> QRAKVAMSHFEPHEYIRYDLLEKNIDIVRKRLNRPLTLSEKIVYGHLDDPANQEIERGKTYLRLRPDRVAMQDATAQMAMLQFISSGLPKVAVPSTIHCDHLIEAQLGGEKDLRRAKDINQEVYNFLATAGAKYGVGFWRPGSGIIHQIILENYAYPGVLLIGTDSHTPNGGGLGGICIGVGGADAVDVMAGIPWELKCPKVIGVKLTGSLSGWTSPKDVILKVAGILTVKGGTGAIVEYHGPGVDSISCTGMATICNMGAEIGATTSVFPYNHRMKKYLSKTGRADIANLADEFKDHLVPDSGCHYDQLIEINLSELKPHINGPFTPDLAHPVAEVGSVAEKEGWPLDIRVGLIGSCTNSSYEDMGRSAAVAKQALAHGLKCKSQFTITPGSEQIRATIERDGYAQVLRDVGGIVLANACGPCIGQWDRKDIKKGEKNTIVTSYNRNFTGRNDANPETHAFVTSPEIVTALAIAGTLKFNPETDFLTGKDGKKFKLEAPDADELPRAEFDPGQDTYQHPPKDSSGQRVDVSPTSQRLQLLEPFDKWDGKDLEDLQILIKVKGKCTTDHISAAGPWLKFRGHLDNISNNLLIGAINSENRKANSVRNAVTQEFGPVPDTARYYKQHGIRWVVIGDENYGEGSSREHRALEPRFLGGRAIITKSFARIHETNLKKQGLLPLTFADPADYNKIHPVDKLTIQGLKDFAPGKPLTCIIKHPNGTQETILLNHTFNETQIEWF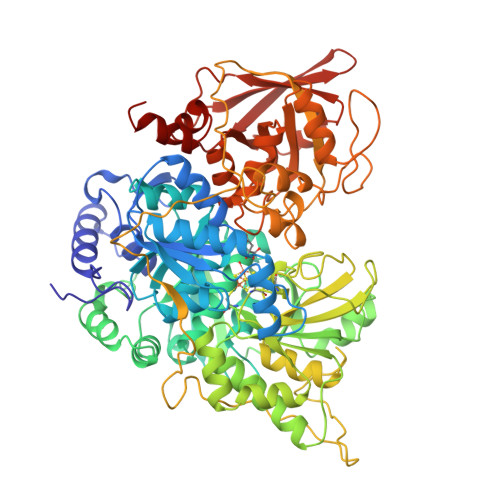RAGSALNRMKELQQK>[10x]MKNKLKVLALTLASLSSVCYANMADYNTYQSNVQINNLSYG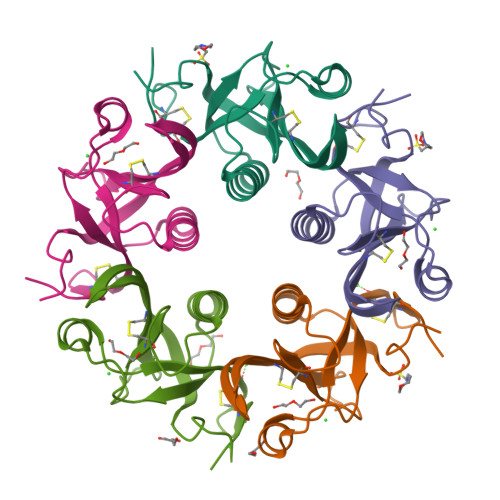VYRSGDKESQFFCVGLKRGSQVPNVHTICKIDVFGTHKQGFDNMLATARYYYATGEDVRIYYKENVWTDRNFTAAFSGNELIAITTCTSSDYCMGPTLPNLEHHHHHH>AUGUGGC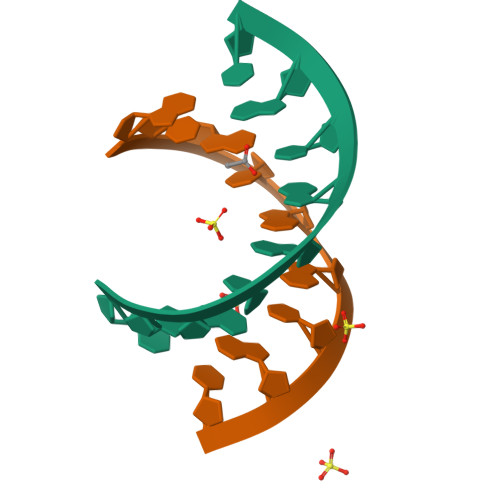AU[2x]5-{[AMINO(IMINO)METHYL]AMINO}PENTANOIC ACID | C6 H13 N3 O2 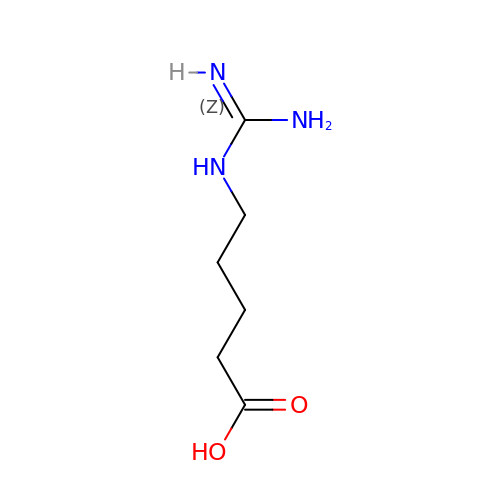| UKUBCVAQGIZRHL-UHFFFAOYSA-N> ASMQKLINSVQNYAWGSKTALTELYGIANPQQQPMAELWMGAHPKSSSRITTANGETVSLRDAIEKNKTAMLGEAVANRFGELPFLFKVLCAAQPLSIQVHPNKRNSEIGFAKENAAGIPMDAAERNYKDPNHKPELVFALTPFLAMNAFREFSDIVSLLQPVAGAHSAIAHFLQVPNAERLSQLFASLLNMQGEEKSRALAVLKAALNSQQGEPWQTIRVISEYYPDDSG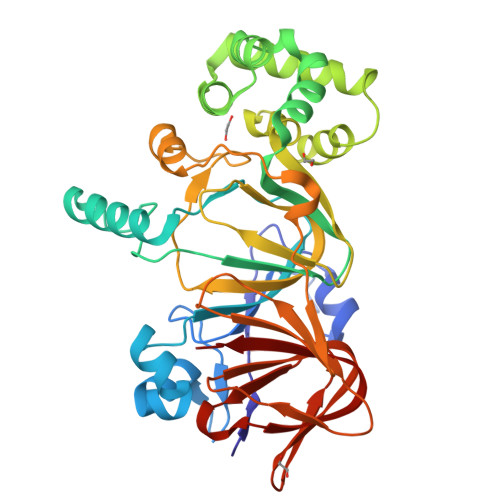LFSPLLLNVVKLNPGEAMFLFAETPHAYLQGVALAVMANSDNVLRAGLTPKYIDIPELVANVKFEPKPAGELLTAPVKSGAELDFPIPVDDFAFSLHDLALQETSIGQHSAAILFCVEGEAVLRKDEQRLVLKPGESAFIGADESPVNASGTGRLARVYNKL3-({4-[(2,4-dimethyl-5-sulfophenyl)amino]-9,10-dioxo-9,10-dihydroanthracen-1-yl}amino)-2,4,6-trimethylbenzenesulfonic 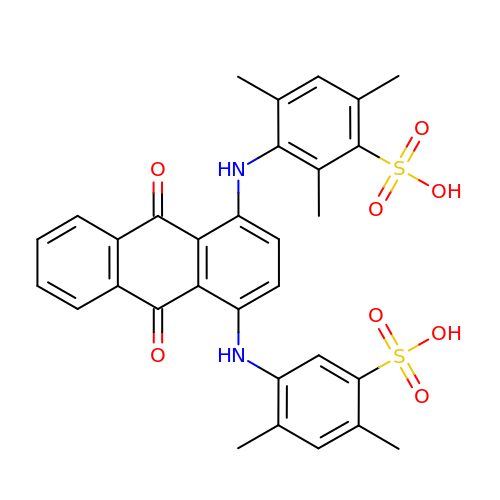acid | C31 H28 N2 O8 S2 | WWMZMGAHGSMSEO-UHFFFAOYSA-N> NETDALKDRIENIRPRMTLAAKLRELMPEIDRQVRAGVQHDDIVETLNANG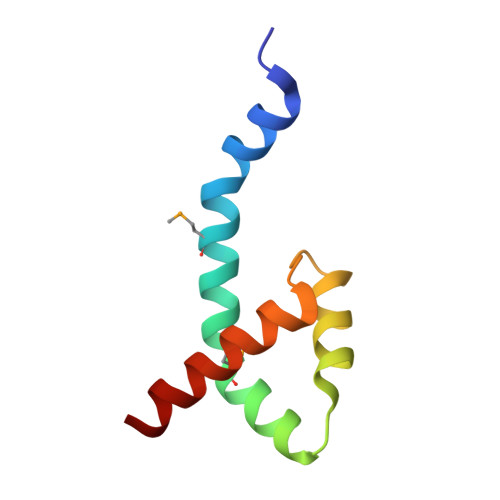FDVNLNTFRSYLYRYRKKARA>[2x]KHPTPMLDELEKGPWPSFVSDIKQECDNRAKNPKGLDYQIPAECPDDLLGILELSFHEGETHWKHGGIVGVFGYGGGVIGRYCDQPEMFPGVAHFHTVRLAQPAAKYYTAEYLEAICDVWDLRGSGLTNMHGSTGDIVLLGTQTPQLEEIFFEMTHNLNTDLGGSGSNLRTPESCL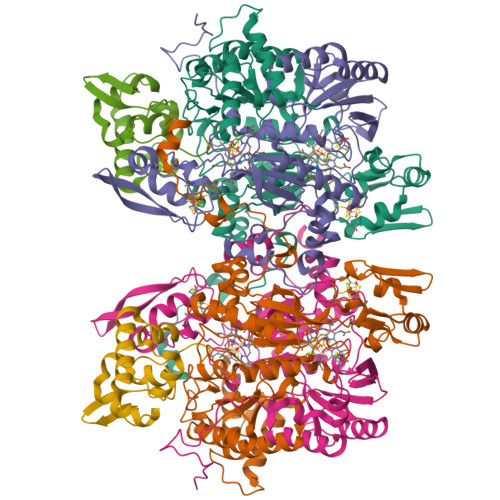GISRCEFACYDTQLMCYQLTQDYQDELHRPAFPYKFKFKFDGCPNGCVASMARSDFAVIGTWKDDIKIDQEAVKAYVGGEFKPNAGAHAGRDWGKFDIEAEVVGLCPTGCMTYESGTLSIDNKNCTRCMHCINTMPRALKIGDERGASILVGAKAPVLDGAQMGSLLIPFIAAEEPFDEVKEVIENIWEWWMEEGKNRERLGETMKRVGFQKLLEVTGTKAVPQHVSEPRHNPYIFFKEEEVPGGWSRDISDYRKRHMR;>AFISSGYNPAKPMENRITDIGPRKFTEFFPPVIAKNAGNWDYHEILEPGILVHVAKNGDKVFTVRCGAARLMSTSHIREACEIAKKFCNGHLRFTTRNNIEFMVDNEETLKALVADLKTRKFAAGSFKFPIGGTGASISNIVHTQGWVYCHTPATDASGPVKAVMDELFEEFTSMRLPAIVRVSLACCINMCGAVHCSDIGLVGIHRKPPMIDHENLAELCEIPLAVAACPTAAVKPITAEVNGQKVKSVAINNDRCMYCGNCYTMCPALPLSDGTGDGIAIMVGGKISNRIKVPSFSKVVVAFVPNEPPRWPTMAKIVKKIVEVYAEDARKYERIGDWIHRIGWETFYEKTGLEFSHHCIDDFRDPAYYTWRQSTQFKFVSFDS[2x];>AVVEFAGSAFEVDEDGFLNAFDDWCPEWVKYAKGSEGIGAGSADHQKIIDFLQDYYKANGIAPMVRILSKVTGFKLKQIYELFPSGPGKGACKMAGLPKPTGCV[2x]SN-GLYCEROL-1-PHOSPHATE 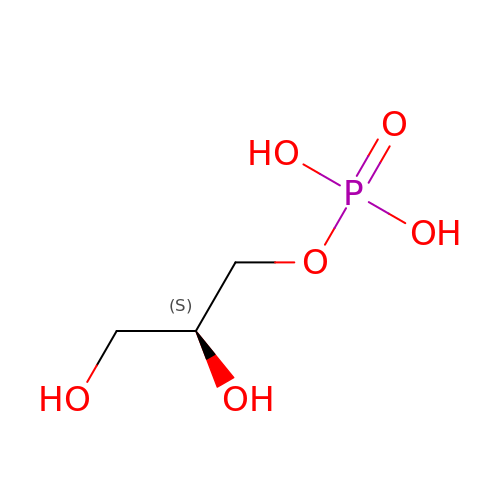| C3 H9 O6 P | AWUCVROLDVIAJX-VKHMYHEASA-N>MSGPAHLPYGGIPTFARAPLVQPDGDWQADVAALGVPFDIALGFRPGARFAPRALREASLRSVPPFTGLDGKTRLQGVTFADAGDVILPSLEPQLAHDRITE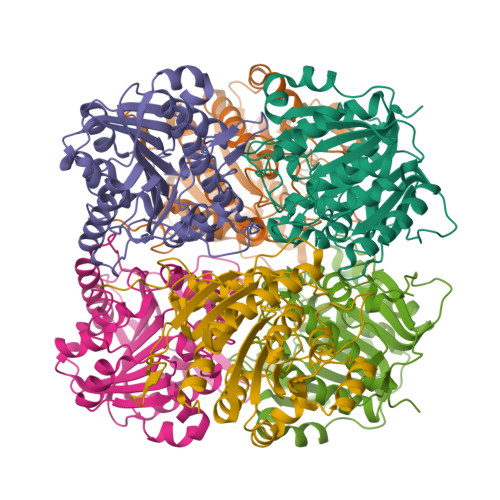AARQVRGRCRVPVFLGGDHSVSYPLLRAFADVPDLHVVQLDAHLDFTDTRNDTKWSNSSPFRRACEALPNLVHITTVGLRGLRFDPEAVAAARARGHTIIPMDDVTADLAGVLAQLPRGQNVYFSVDVDGFDPAVIPGTSSPEPDGLTYAQGMKILAAAAANNTVVGLDLVELAPNLDPTGRSELLMARLVMETLCEVFDHVL[6x]> MARGLNQVFLIGTLTARPDMRYTPGGLAILDLNLAGQDAFTDESGQEREVPWYHRVRLLGRQAEMWGDLLEKGQLIFVEGRLEYRQWEKDGEKKSEVQVRAEFIDPLEGRGRETLEDARGQPRLRRALNQVILMGNLTRDPDLRYTPQGTAVVRLGLAVNERRRGQEEERTHFLEVQAWRELAEWASELRKGDGLLVIGRLVNDSWTSSSGERRFQTRVEALRLERPTRGPAQAGGSRP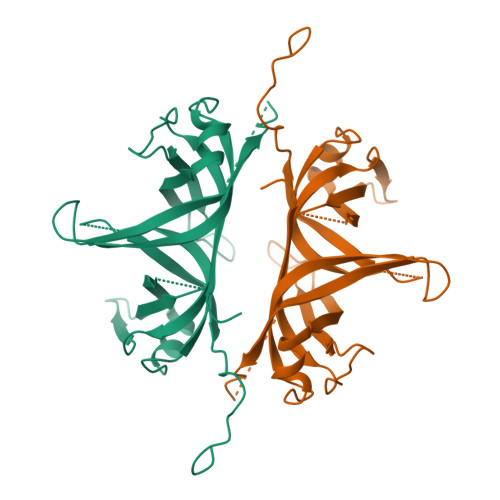PTVQTGGVDIDEGLEDFPPEEDLPF> MPSVIVVGGQWGDEGKGSIVAYLSLHDEPEIIARGGVGTNAGHSVVINGKKYAVRQIPTGFMQTKARLLIGAGVLVDPEVFFHELEQLKDFNVKDRVGIDYRCAIIEEKHKQLDRTNGYLHGKIGTTGSGCGPANADRVMRKAKQAK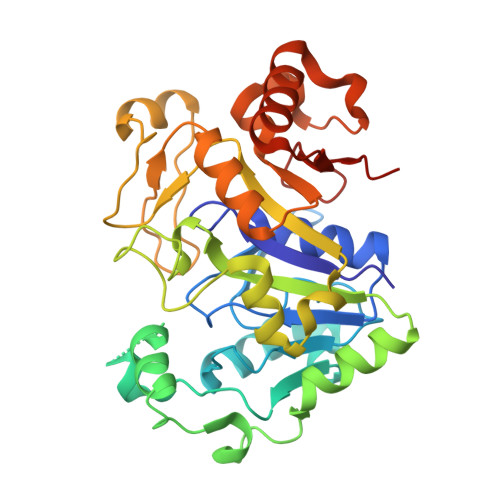DVKELEPYLTDVAQEINDALDEGSLVLVEGTQGFGLSLYYGTYPYVTSKDVTASSVAADVGIGPTRVDEVIVVFKSFPTRVGAGPFPTEMPMEEADRLGLVEYGTVTGRRRRVGWFDFEMARYSARINGATMLAVTMLDKYDKEAFGVTDYDKLPRKAKEFIEEIEERVGVPVGLIKTGPELEHIIDRRDTI> KVQPSPTVHTKEALGFIMNMFQAP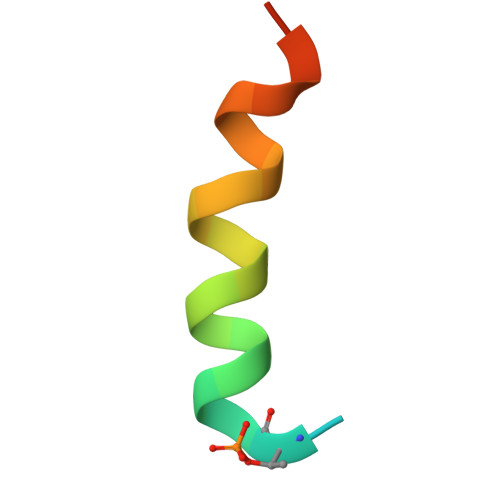TS>MANKQDLIAEVAAKTGLTKKDSEKAVNAFGEVVTEFLAKGEKVQLIGFGTFETRERAAREGR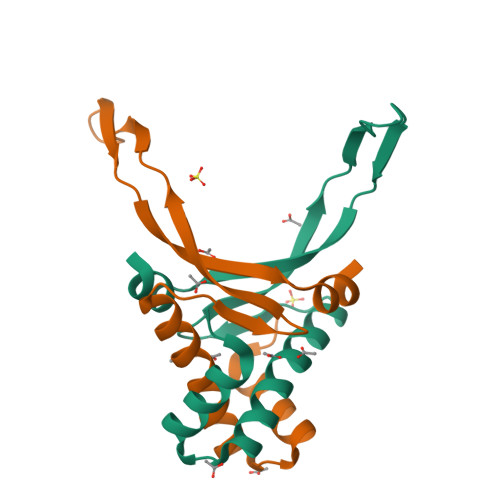NPQTGEAIKIAATVVPAFKAGKALKDAVK[4x]4-[4-[2-(2,4-dichlorophenyl)-4-methyl-5-(piperidin-1-ylcarbamoyl)pyrazol-3-yl]phenyl]but-3-ynyl nitrate | C26 H25 Cl2 N5 O4 | 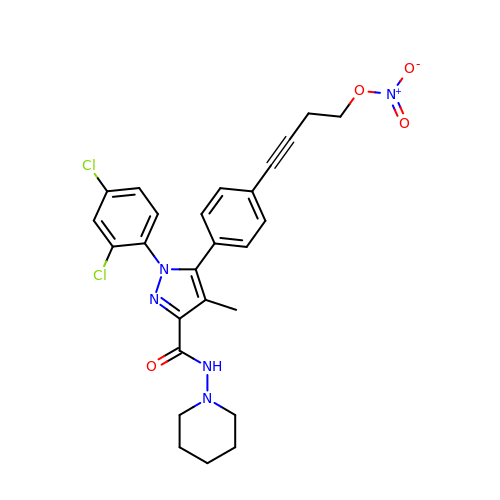KXXKUWQMQUYUSE-UHFFFAOYSA-N>[4x]MIRVACVGITVMDRIYYVEGLPTESGKYVARNYTEVGGGPAATAAVAAARLG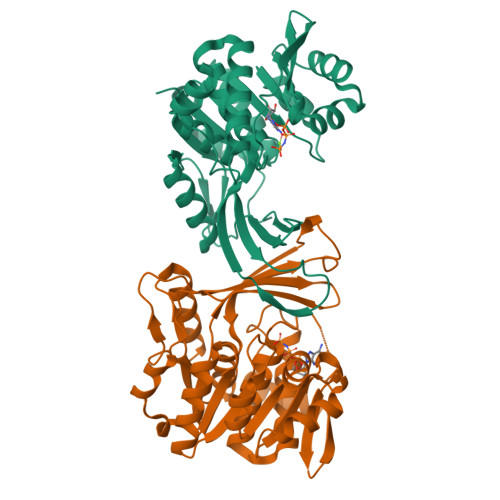AQVDFIGRVGDDDTGNSLLAELESWGVNTRYTKRYNQAKSSQSAIMVDTKGERIIINYPSPDLLPDAEWLEEIDFSQWDVVLADVRWHDGAKKAFTLARQAGVMTVLDGDITPQDISELVALSDHAAFSEPGLARLTGVKEMASALKQAQTLTNGHVYVTQGSAGCDWLENGGRQHQPAFKVDVVDTTGAGDVFHGALAVALATSGDLAESVRFASGVAALKCTRPGGRAGIPDCDQTRSFLSLFVLEHHHHHH>[4x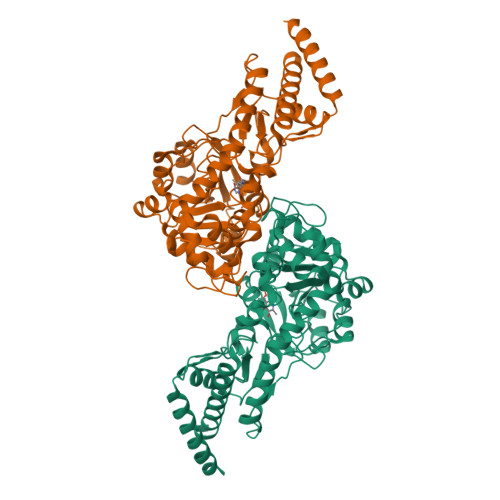]VSFDSLSPQELAALHARHQQDYAALQGMKLALDLTRGKPSAEQLDLSNQLLSLPGDDYRDPEGTDTRNYGGQHGLPGLRAIFAELLGIAVPNLIAGNNSSLELMHDIVAFSMLYGGVDSPRPWIQEQDGIKFLCPVPGYDRHFAITETMGIEMIPIPMLQDGPDVDLIEELVAVDPAIKGMWTVPVFGNPSGVTYSWETVRRLVQMRTAAPDFRLFWDNAYAVHTLTLDFPRQVDVLGLAAKAGNPNRPYVFASTSKITFAGGGVSFFGGSLGNIAWYLQYAGKKSIGPDKVNQLRHLRFFGDADGVRLHMLRHQQILAPKFALVAEVLDQRLSESKIASWTEPKGGYFISLDVLPGTARRTVALAKDVGIAVTEAGASFPYRKDPDDKNIRIAPSFPSVPDLRNAVDGLATCALLAATETLLNQGLASSAPNVR C2-HYDROXY-COELENTERAZINE | C26 H21 N3 O4 | 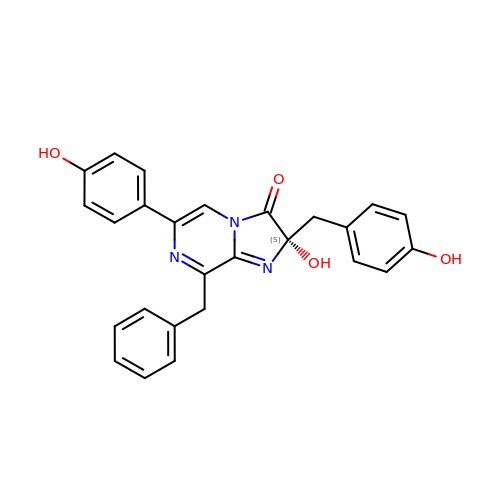ULLMMKZQNNBLRN-SANMLTNESA-N> GGGUGUGUACCGUUCAACUCGUC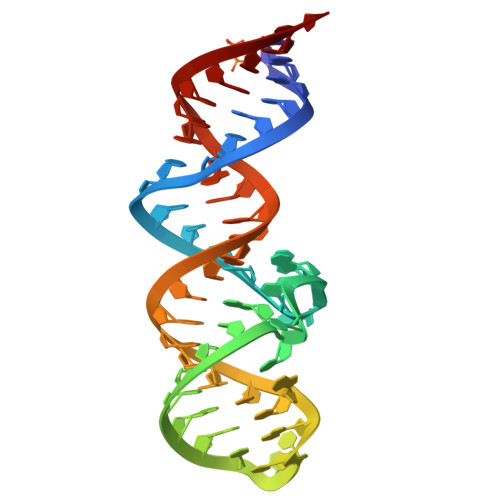CCAGCUUCGACUGGGACUACGGGAGCGCCU>GSHMEPIEEATKCYDQMLIVERYERVISYLYPIAQSIPRKHGVAREMFLKCLLGQVELFIVAGKSNQVSKLYAADAGLAMLRFWLRFLAGIQKPHAMTPHQVETAQVLIAEVGRILGSWIARVNRKG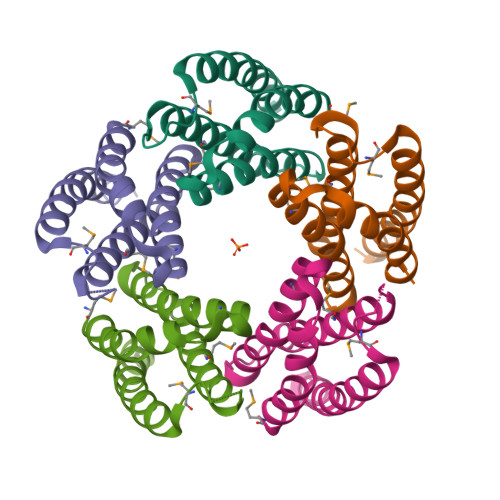QAGK[5x]> LVPRGSAMGISNDSSRGANRTIVVTTILESPYVMYKKNHEQLEGNERYEGYCVDLAYEIAKHVRIKYKLSIVGDGKYGARDPETKIWNGMVGELVYGRADIAVAPLTITLVREEVIDFSKPFMSLGISIMIKKGTPIESAEDLAKQTEIAYGTLDSGSTKEFFRRSKIAVYEKMWSYMKSAEPSVFTKTTADGVARVRKSKGKFAFLLES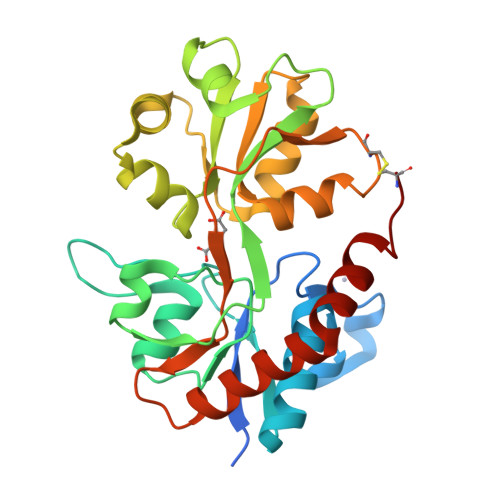TMNEYIEQRKPCDTMKVGGNLDSKGYGVATPKGSALGTPVNLAVLKLSEQGILDKLKNKWWYDKGECG>[2x]VNGAGLLQTVWGPVCELTSELDGQAGAALKKEQEMLAKINDMQMAQLRAAIYLAKNPSTPHQNALAVLTAYYAERAGSGKAYFLHALPKAVDSIRRAAYLKGHLDEYLNLLEKSSGGNNKCLVTTDDATVATRGGDQKLAGKNCKLSLSPLKPVDAALTYITKAGVGKLRYDDGGAGGNAVTPSKSGVHACKLLIAHNTAGYGDGGGVTADIDVFA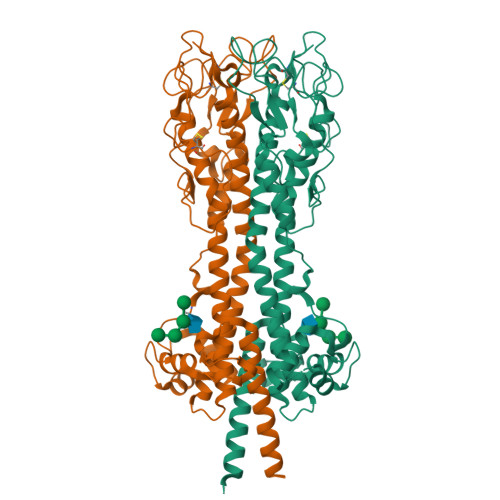GYMKVKATDAEPKLAAKSDLEEGGGGGAEAWKALHTAIKQEADAEAAELTNETGKLGERRHFLAAATNVLGTGAAGTGNAGRAAVEAAFGSDSEGGDRKIIELIEKELIVKGTANRDADESLGNIKTLKELGELLSYFQLKNSNTINELRNKLKA;>[3x]VNGAGLLQTVWGPVCELTSELDGQAGAALKKEQEMLAKINDMQMAQLRAAIYLAKNPSTPHQNALAVLTAYYAERAGSGKAYFLHALPKAVDSIRRAAYLKGHLDEYLNLLEKSSGGNNKCLVTTDDATVATRGGDQKLAGKNCKLSLSPLKPVDAALTYITKAGVGKLRYDDGGAGGNAVTPSKSGVHACKLLIAHNTAGYGDGGGVTADIDVFAGYMKVKATDAEPKLAAKSDLEEGGGGGAEAWKALHTAIKQEADAEAAELTNETGKLGERRHFLAAATNVLGTGAAGTGNAGRAAVEAAFGSDSEGGDRKIIELIEKELIVKGTANRDADESLGNIKTLKELGELLSYFQLKNSNTINELRNKLK;>[3x]VNGAGLLQTVWGPVCELTSELDGQAGAALKKEQEMLAKINDMQMAQLRAAIYLAKNPSTPHQNALAVLTAYYAERAGSGKAYFLHALPKAVDSIRRAAYLKGHLDEYLNLLEKSSGGNNKCLVTTDDATVATRGGDQKLAGKNCKLSLSPLKPVDAALTYITKAGVGKLRYDDGGAGGNAVTPSKSGVHACKLLIAHNTAGYGDGGGVTADIDVFAGYMKVKATDAEPKLAAKSDLEEGGGGGAEAWKALHTAIKQEADAEAAELTNETGKLGERRHFLAAATNVLGTGAAGTGNAGRAAVEAAFGSDSEGGDRKIIELIEKELIVKGTANRDADESLGNIKTLKELGELLSYFQLKNSNTINELRNKLKAV The multifunctional adaptor protein SLy1 (SH3 domain-containing protein expressed in lymphocytes 1), also known as SASH3 (SAM and SH3 domain containing protein 3), is exclusively expressed in lymphocytes and plays different roles in various lymphocyte subsets. SLy1 is 380 amino acids in length and contains a bipartite nuclear localization signal (NLS), a Src homology 3 (SH3) and a sterile alpha motif (SAM) domain, which makes SLy1 a prototypical adaptor protein. In the current report, we show that the SAM domain of SLy1 self-associates to form a distinct dimer with an affinity much stronger than reported previously for homodimerization of other SAM domains. Structure determination reveals that this SAM domain forms a novel type of dimer interface that is incompatible with homooligomerization.

The first variant is referred to as SAMwt and contains the SAM domain (P254–Y316), the five residues D317-E321 succeeding it in SLy1, and an N-terminal glycine from the tag. In parallel, we determined the crystal structure of SAMwt to a resolution of 2.05 Å. The structure belongs to the tetragonal space group P 41 21 2 with one molecule in the asymmetric unit. The final structure comprised 65 of the expected 69 residues (P254–D317 plus the N-terminal glycine). No electron density was visible for T318–E321 in the weighted 2Fo-Fc map, most likely because of conformational flexibility at the termini. The 3D-structure adopts the typical five helix bundle of a SAM domain with the following secondary structure elements: α1 (L257–R263), α3 (L281–F284), α4 (E289–E294) and α5 (P300–Y316). In addition, a composite helix c2 (E267–L274) was identified consisting of a 310-helix (E267–H269) and an α-helical segment (T270–L274). The highest dissociation free energy was obtained for a crystallographic dimer with 2-fold crystallographic symmetry in which helices α5 and α5′ point in the same direction and are located in close proximity to each other. A free energy gain of 4.7 kcal mol−1 and a buried surface area of ~870 Å2 upon SAMwt symmetric dimer formation were obtained. Hydrogen bonds and salt bridges between amino acids in helices α1 and α5′ and between P300 and Q301 at the N-terminus of helices α5 and α5′, respectively, stabilize the dimer interface.

> GPKTLHELLERIGLEEHTSTLLLNGYQTLEDFKELRETHLNELNIMDPQHRAKLLTAAELLLDYD>MRLSYEALEWRTPIENSTEPVSLPPPPPFFGQERAREALELAIRGGFHAYLVGPPSLGKHEALLAYLSTQSVETPPDLLYVPLSERKVAVLTLPSGQEIHLAEAVEGLLLEVNRLDELFRQGSFLREKTQLEARFKEAREQQLEALRREAQEAGFALSTNGERLELTGPGPVPAELSARLEEVTLGSLAASAELEVALRRLRRDWALHYLNNRFEPLFQRFPQARAYLEALRARLARYAETGEPLDPAQWRPNLLTSSSSGTPPPIVYEPYATAPRLFGRLDYLVDRGVWSTNVSLIRPGAVHRAQGGYLILDALSLKREGTWEAFKRALRNGQVEPVTEPQAPAGLEVEPFPIQMQVILVGTPEAFEGLEEDPAFSELFRIRAEFSPTLPASPENCTALGGWLLAQGFQLTQGGLTRLYDEARRMAEQRDRMDARLVEIRALAEEAAVLGGGLLTAESVEQAIAAREHRSFLSEEEFLRAVQEGVIRLRTTGRAVGEVNSLVVVEAAPYWGRPARLTARAAPGRDHLISIDR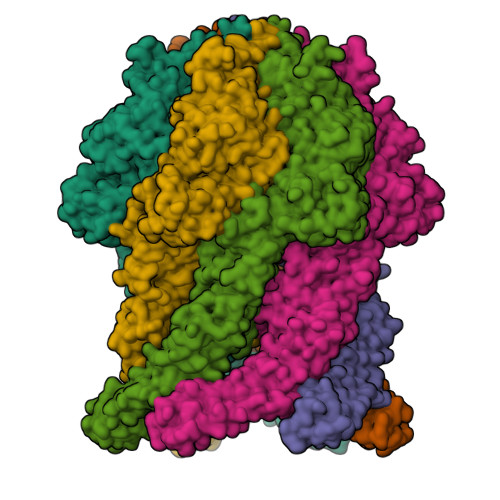EAGLGGQIFHKAVLTLAGYLRSRYIEHGSLPVTISLAFEQNYVSIEGDAAGLAELVAALSAIGNLPLRQDLAVTGAVDQTGKVLAVGAINAKVEGFFRVCKALGLSGTQGVILPEANLANLTLRAEVLEAVRAGQFHIYAVETAEQALEILAGARMEGFRGLQEKIRAGLEAFARLEEGHDKEDREKLAAALEHHHHHH[6x]>[12x]MERELPIPVFLTEDEDSVHERMLSNFQDVSTLEGDFIYDATRPTAEQIAELKQLGLQNNLKIAFPQTSYGTYLEWLGECKGVFKNQPTKATGVITFTGVQGTIITKGTIVTTIATDEKQSIEFELLETKTIGENETVDIKAESRIVGTIGNVSKGSISVLLGSISGVKSITNKEDFRGGTDIEDEEHFRERVLVAEQEDKLSGASSDYIR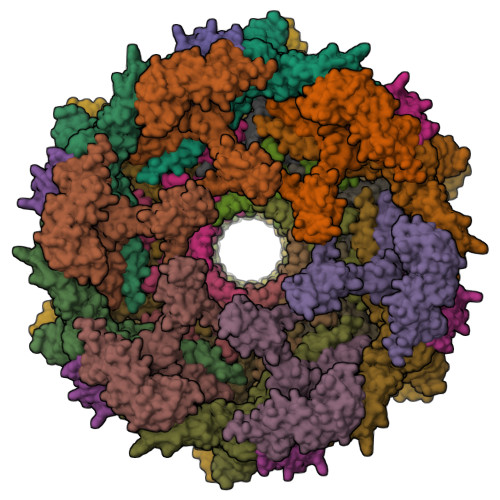WAKEVDGVGYAYVVSEWAGAGTVKVLILDKNRKAATQELIDKVQEYIYPLNISEGENRDGKAPIGALVTVVTPDTLLINVKASFIFSNGFSEETVLNNLKTKIDKYLDKIDLGGTVSYNAIQAIVGSMMLTDEGIEDFSNLTINDVKENIKLQDQVVGIGEIVNEVVG;>MIASKKGKEMLLTLSPIYEQSIIMQSLYEAIGSEFDNLELLDEEIELQLFPQSATWGLGFWENRVGLITNLDEDMETRRRKVIAKLQSKYIMTPKRMSMILQSYTGANIKINENISPYTFGVELTSTQGFPKDLEDLYKRVNVIKPSHLAVSYKLVSLLKSKTYFAQTAIMSEEITIYPYTSKEVKASVKAKFALAHNMSSETLTVYPR[6x];>[6x]MVIDIYLKNEKEKIDFHFPVNPQDSLSIKKEKRFETVDIVNLGEFDIKKEGEKIREISFKTFLPNLYDASYCRYSELKNPIEVVAMLEKWVDQAEPLRLIITGFGYNGLVTISSFSNTQTAGREEDRDIEITFRTYRELKIETLKKDTKSNTKTDLKDNRPNTQTKSKIYTVKASDTLYKIAKNLLGKGSRWPEIYNIPENKKVIGKNPNIIKKGQKLVIPSK;>[6x]MYNDDYIEEASFLNGSDVVILIDGVEELYMEEIKADFEQDEQSIKLLGCQNEISRVGTTKGSFSLNGYKTDSKFAKLGFRSFEIIYNLSNSETLGYESIRLKNCRLKKLPLINSKAGEIVKIEVEGSFRGYDLLNEL;>MATGTWNEKERKEIPGFYNRFKTQAEKSTNTGLKGRLAMPIRANWGDVGKVVTIKNDLRQLKNLFGDDMNYSAFKLGKLALLGNVKELLLYRLVDGNQKKGTLTLKDTTENSAKDVIKLETKYPTARNFNVTIKSNLVDSDKKDFIFFENTKQLFSSSIKGTIDEIVLEINSNLDNEYVIATKVADSDTILANVVNQALEGGNDGCTSITNESYLKALEEFERYSFDSFVLDGVADEALQETTKAWVAKNKELGKDILLFLGGKTEDNIKQINDKSKSFNDENIVNVGSSAYYENIKYTPSEVAVYIAALSVSKGITGSICNAKTIFEEVEPRLSQSEVKECLKSGTLVLDFDDGDVIIVDDVNTFKKYVDDKNEAMGYISNIMFINTINKDTSLKRKEFVGKIFNDATGQTTVICALKKYFEELMSQGIISEFNVDIDTELQATAKADEFYWKWDAVKVDVMKKIYGTGYLG[6x];>[6x]MPNLFPQSETFETVELKNNDENELDLKGSFLFDFEKGEFVKNADGTLKKCDKVQAYKQWCQKAILTPRYKKAAYTNIYGSEIKDLIASNLSQSAKELEITRLIKETILVHPYTKEVGEFSFNWLENSRLVEYEFDVLTIDDENIVIDGNIKR> YKEEDSTVSILPTSLPQIHRANMLAQGSPAASKISPLVTKKSKTRWHFGIRSRSYPLDVMGEIYIALKNLGAEWAKPSEEDLWTIKLRWKYDIGNKTNTNEKIPDLMKMVIQLFQIETNNYLVDFKFDG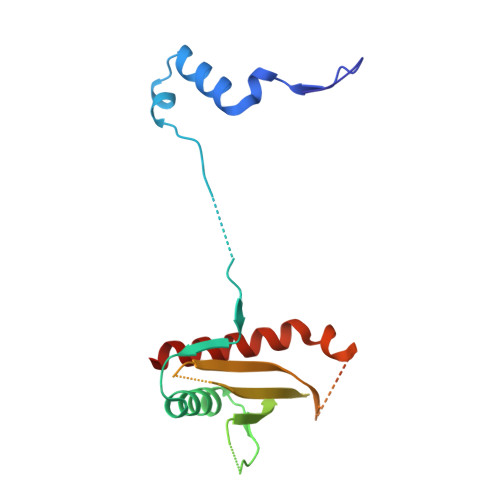WESSYGDDTTVSNISEDEMSTFSAYPFLHLTTKLIMELAVNS>[2x]HMRVLVVPLPYPTHLMAMVPLCWALQASGHEVLIAAPPELQATAHGAGLTTAGIRGNDRTGDTGGTTQLRFPNPAFGQRDTEAGRQLWEQTAS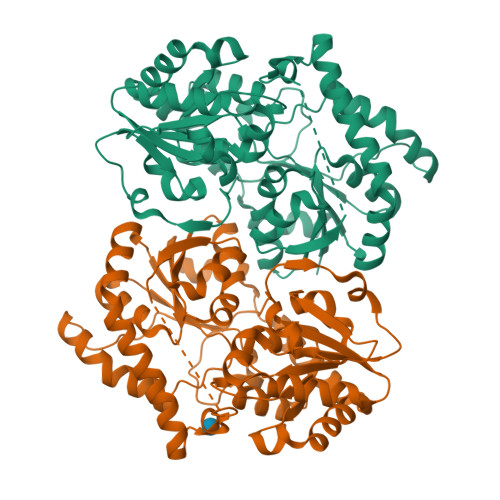NVAQSSLDQLPEYLRLAEAWRPSVLLVDVCALIGRVLGGLLDLPVVLHRWGVDPTAGPFSDRAHELLDPVCRHHGLTGLPTPELILDPCPPSLQASDAPQGAPVQYVPYNGSGAFPAWGAARTSARRVCICMGRMVLNATGPAPLLRAVAAATELPGVEAVIAVPPEHRALLTDLPDNARIAESVPLNLFLRTCELVICAGGSGTAFTATRLGIPQLVLPQYFDQFDYARNLAAAGAGICLPDEQAQSDHEQFTDSIATVLGDTGFAAAAIKLSDEITAMPHPAALVRTLENTAAIRA(3S)-3-aminopyrrolidin-2-one | C4 H8 N2 O | 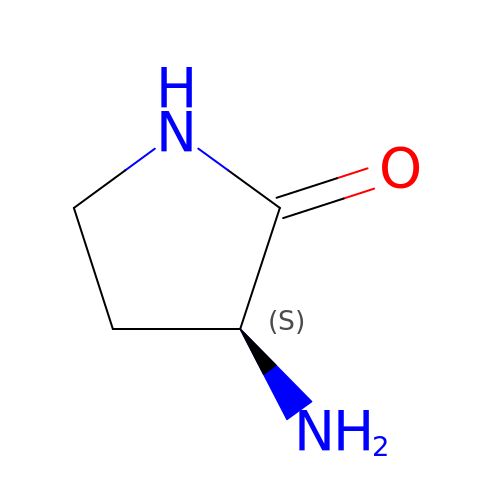YNDAMDVOGKACTP-VKHMYHEASA-N> MNSPISPIETVPVKLKPGMDGPKVKQWPLTEEKIKALVEICTEMEKEGKISKIGPENPYNTPVFAIKKKDSTKWRKLVDFRELNKRTQDFWEVQLGIPHPAGLKKKKSVTVLDVGDAYFSVPLDEDFRKYTAFTIPSINNETPGIRYQYNVLPQGWKGSPAIFQSSMTKILEPFRKQNPDIVIYQYMDDLYVGSDLEIGQHRTKIEELRQHLLRWGLTTPDKKHQKEPPFLWMGYELHPDKWTVQPIVLPEKDSWTVNDIQKLVGKLNWASQIYPGIKVRQLCKLLRGTKALTEVIPLTEEAELELAENREILKEPVHGVYYDPSKDLIAEIQKQGQGQWTYQIYQEPFKNLKTGKYARMRGAHTNDVKQLTEAVQKITTESIVIWGKTPKFKLPIQKETWETWWTEYWQATWIPEWEFVNTPPLVKLWYQLEKEPIVGAETFYVDGAANRETKLGKAGYVTNRGRQKVVTLTDTTNQKTELQAIYLALQDSGLEVNIVTDSQYALGIIQAQPDQSESELVNQIIEQLIKKEKVYLAWVPAHKGIGGNEQVDKLVSAGIRKVL;> MAGHHHHHHGSAENLYFQGPISPIETVPVKLKPGMDGPKVKQWPLTEEKIKALVEICTEMEKEGKISKIGPENPYNTPVFAIKKKDSTKWRKLVDFRELNKRTQDFWEVQLGIPHPAGLKKKKSVTVLDVGDAYFSVPLDEDFRKYTAFTIPSINNETPGIRYQYNVLPQGWKGSPAIFQSSMTKILEPFRKQNPDIVIYQYMDDLYVGSDLEIGQHRTKIEELRQHLLRWGLTTPDKKHQKEPPFLWMGYELHPDKWTVQPIVLPEKDSWTVNDIQKLVGKLNWASQIYPGIKVRQLCKLLRGTKALTEVIPLTEEAELELAENRE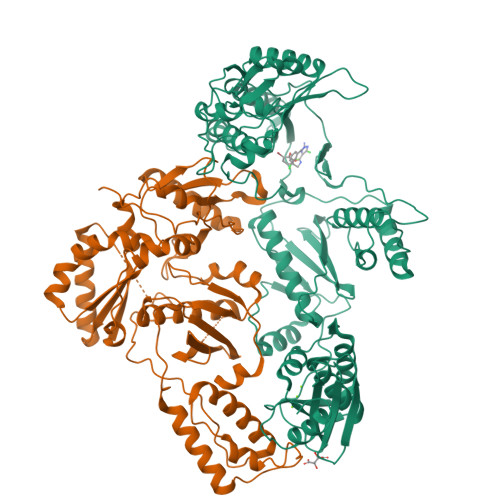ILKEPVHGVYYDPSKDLIAEIQKQGQGQWTYQIYQEPFKNLKTGKYARMRGAHTNDVKQLTEAVQKITTESIVIWGKTPKFKLPIQKETWETWWTEYWQATWIPEWEFVNTPPLVKLWYQ>HTRTLGFILPDLENPSYARIAKQLEQGARARGYQLLIASSDDQPDSERQLQQLFRARRCDALFVASCLPPEDDSYRELQDKGLPVIAIDRRLDPAHFCSVISDDRDASRQLAASLLSSAP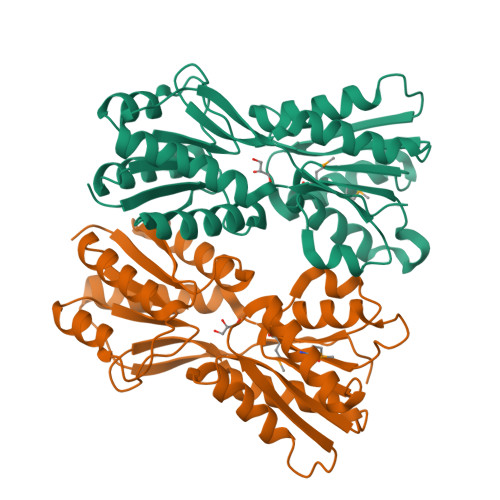RSIALIGARPELSVSQARAGGFDEALQGYTGEVRRYQGEAFSRECGQRLMQQLIDDLGGLPDALVTTSYVLLQGVFDTLQARPVDSRQLQLGTFGDNQLLDFLPLPVNAMAQQHGQIAATALELALAAIEEKRYEPGVHAVGRTFKQRISVA[2x]> GPGSMKRNRVVIFISGGGSNMEALIRAAQAPGFPAEIVAVFSDKAEAGGLAKAEAAGIATQVFKRKDFASKEAHEDAILAALDVLKPDIICL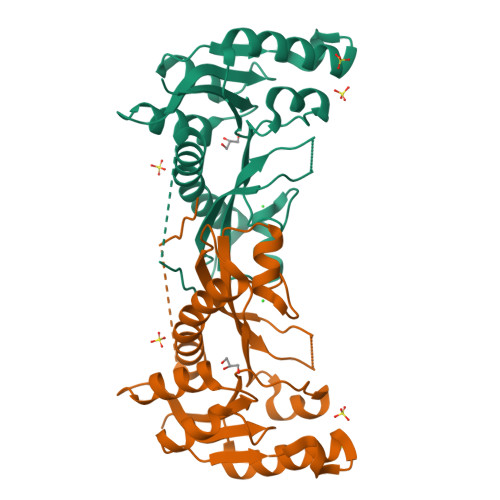AGYMRLLSGRFIAPYEGRILNIHPSLLPLFPGLHTHQRALDAGMKLAGCTVHLVTEGMDEGPILAQAAVPVLDGDTAETLAARVLKAEHRLYPLALQKFAAGEKASNQFSDGMVLSA>[3x]MAIKNAFYAQSGGVTAVINASACGVIQTARKHPDQIGKVYAGRNGIIGALKEELIDTSLESDDAIQALIHTPGGAFGSCRYKLKNISENQREYERLIEVFRAHDIGYFFYNGGGDSQDTAYKVSQLADRMGYPITCIGVPKTVDNDLPFTDCCPGFGSVAKYIATSTLEASLD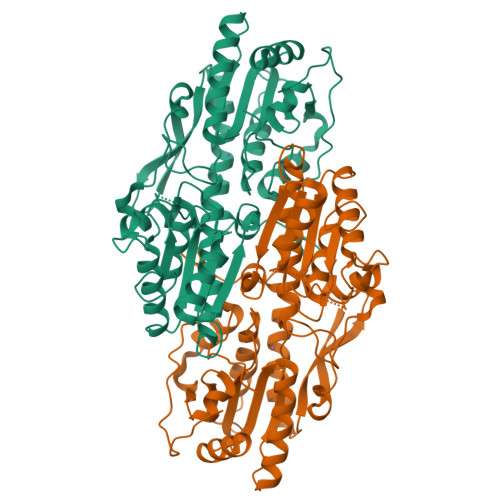IKSMCETSTKVFILEVMGRHAGWIAAAGGLAGQSEGEPPHVILFPEIPFNREKFLERVDQCVRDYGYCVVVASEGAQYEDGRFVADAGAKDAFGHTQLGGVAPALANMVKQALGHKYHWAVADYLQRAARHIASATDVEQAYAVGKAAVEMALAGKQALMPTIVRDQAKPYRWSIGEANLSEVANQEKKMPIHYITDNGFGITQDCRDYLQPLIAGESFPPFDDGLPRVAKLKNQLVEKKLRTEFEL Botulinum neurotoxin (BoNT) is the active agent that causes the deadly condition botulism. The smaller 50 kDa light chain (LC) possesses a single zinc-endopeptidase domain whereas the larger 100 kDa heavy chain is comprised of two domains—a target cell receptor binding (HC) domain and a translocation (HN) domain. The BoNT HC domain is responsible for targeting the toxin to a specific cell type and the specific receptors involved have been identified for most serotypes. As with all reported structures of the BoNT receptor binding domain, present is a characteristic β-jellyroll fold at the N-terminal half and a predominantly β-trefoil fold at the C-terminal half of the protein.

Recently, a new bivalent strain of Clostridium botulinum, IBCA10-7060, was reported to produce BoNT/B2 and a previously unknown BoNT serotype—“BoNT/H”. This novel toxin is a mosaic molecule and is now more commonly referred to as BoNT/FA (as well as BoNT/HA) due to a LC similar to that of BoNT/F5, a HN domain similar to that of BoNT/F1, and a HC domain similar to that of BoNT/A1. Here, we present a new crystal structure of HC/FA at 1.95 Å resolution which reveals further structural information that is unresolved in the reported structure. Specifically, our structure reveals a loop previously unmodeled due to lack of density, which is of high importance, and we also observe a disulphide bond which was not present within the previous structure. We identified crystallisation conditions which yielded crystals of HC/FA in space group P422, with two molecules related by non-crystallographic symmetry in the asymmetric unit. However, it further reveals the presence of a loop (R1261–R1268) that has been shown in other subtypes to be involved in ganglioside receptor binding. Crystal packing has enabled neighbouring chains to interact directly with this loop, provide sufficient stabilisation to produce good electron density. Yao et al. (2017) suggested that the lack of density was due to high flexibility, which is consistent with the high B-factors we observed in this region relative to the rest of the protein. The specific ganglioside receptor for BoNT/FA is not yet known; however, considering that GT1b binds with high affinity to BoNT/A1 and that HC/FA and HC/A1 are structurally very similar, we propose that BoNT/FA possesses a similar binding specificity.

>MHHHHHHGELKYNCILNIKYEMDRDKLVDSSGYRSRINIGTGVKFSEIDKNQVQLSNLESSKIEVILNNGVIYNSMYENFSTSFWIRIPKYFRNINNEYKIISCMQNNSGWEVSLNFSNMNSKIIWTLQDTEGIKKTVVFQYTQNINISDYINRWIFVTITNNRLSNSKIYINGRLINEESISDLGNIHASNNIMFKLDGCRDPHRYIWIKYFNLFDKELNKKEIKDLYDNQSNSGILKDFWGDYLQYDKPYYMLNLYDPNKYLDVNNVGIRGYMYLKGPRGRIVTTNIYLNSTLYMGTKFIIKKYASGNKDNIVRNNDRVYINVVVKNKEYRLATNASQAGVEKILSAVEIPDVGNLSQVVVMKSENDQGIRNKCKMNLQDNNGNDIGFIGFHQFNNIAKLVASNWYNRQIGKASRTFGCSWEFIPVDDGWGESSL[2x]>GGGRNPPEGASEEGGAADSDVDAFFRTGSFRNDGLKASDVLPILKEKVAFVSGGRDKRGGPILTFPARSNHDRIRQEDLRKLVTYLASVPSEDVCKRGFTVIIDMRGSKWDLIKPLLKTLQEAFPAEIHVALIIKPDNFWQKQKTNFGSSKFIFETSMVSVEGLTKLVDPSQLTEEFDGSLDYNHEEW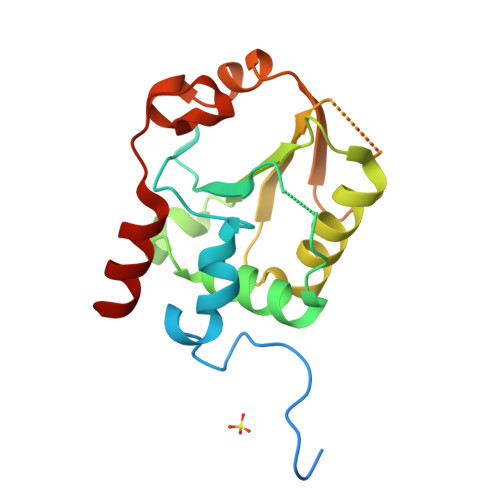IELRLSL[8x]>YFGKLESKLSVIRNLNDQVLFIDQGNRPLFEDMTDSDCRDNAPRTIFIISMYKDSQPRGMAVTISVKCEKISTLSCENKIISFKEMNPPDNIKDTKSDIIFFQRSVPGHDNKMQFESSSYEGYFLACEKERDLFKLILAAADAAG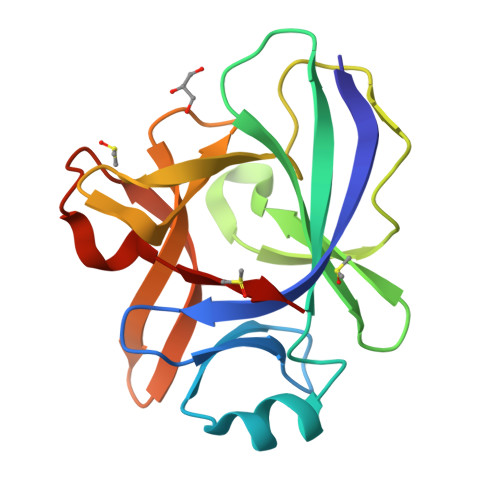DRSIMFTVQNED[2x]> DRHHHHHHGSRSSLNDDLLSPYQPHAKHGPSHSYRHVRDSQPVIHGNRTHEEWPSSNSTWMPVATTRIFESKFPTTSGMKTAYGHFTYVNNPLRTFSVLEPGGPGGCSKKLTATVEETIKHGNCFVAQNGGYFDMDTGNCFGNIVSDGKLVQSAKGIQNAQFGIKSDGTLIFGYLSEEQVLEAENPFVQLLSGVVWLLRNGEVYINQSKAAESDKTQTTGDFDHFINVISARTAIGHDREGRLIIFHVDGQTDDRGLNLWELANFLKDQGVINAINLDGGGSATLVINGTLANYPSDHCHYNPMWRCPRSISTVVCVHEPFCDPPDCSGHGQCILGECQCTDFWTGPACSVLSCGPLNCSAHGNCTEGGCVCDQGWIGADCNISCVHGYYGEGCRR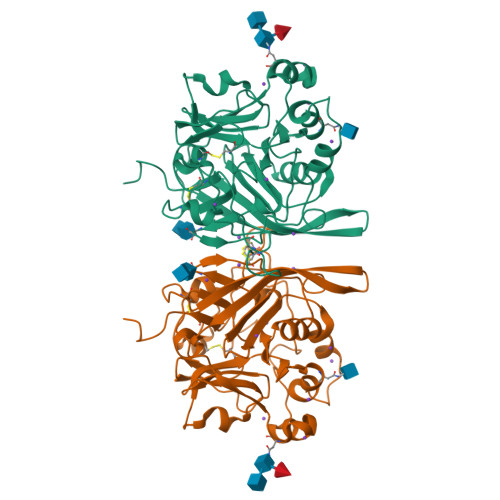KCPCQNNSTCNHVDGSCQCSDGYTGLYCEEECPLGFYGAGCQHACHCKNQSYCDHLTGSCNITKKPSLNELSSKVGQSMETLLSTSLKNTRHSETAVNIFA>SNAMSRDLGRLLKIASNQMSTRFDIFAKKYDLTGTQMTIIDYLSRNKNKEVLQRDLESEFSIKSSTATVLLQRMEIKKLLYRKVSGKDSRQKCLKLTKKANKLETIILSYMDSDQSQMTSGLNKEEVVFLEKILKRMI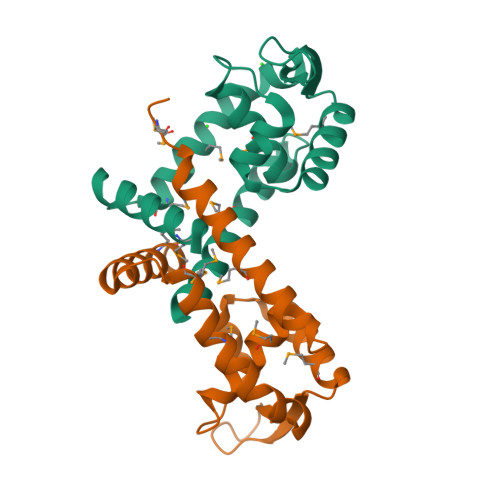ESD[4x]>GHMEQTHRAIFRFVPRHEDELELEVDDPLLLELQAEDYWYEAYNMRTGARGVFPAYYAIEVTK[12x]

Aromatic residues cluster in the core of folded proteins, where they stabilize the structure through multiple interactions. NMR studies in the 1970s demonstrated that aromatic side chains can undergo ring flips—that is, 180° rotations of the χ2 dihedral angle (Cβ–Cγ axis)—even when engaged in stabilizing interactions in the hydrophobic core. Here we capture ring flipping events of a buried tyrosine residue in the SH3 domain of the JNK-interacting protein 1 (JIP1). Our data therefore suggest that the conformation of the aromatic ring at position 526 is determined by steric interactions dictated by the size of the surrounding amino acids.

The PCA suggests that a staggered conformation in group 2 is favoured over an eclipsed conformationin group 1 when residues with larger side chains are found in position 541, when isoleucine or leucine are occupying position 517 and when smaller residues are found in position 493. Accordingly, we designed four different mutants of JIP1-SH3 (H493A, V517A, V517L and A541L) and obtained their high-resolution structures by X-ray crystallography. Of note, three mutants (H493A, V517A and A541L) induce a staggered conformation of Y526, with χ2 dihedral angles ranging from −41° to −75°, whereas V517L shows an eclipsed conformation of Y526 and an almost identical structure to the wild-type protein. The high resolution of these structures, ranging from 1.4 to 1.9 Å, allows unambiguous determination of the conformation of Y526 and the surrounding residues, as demonstrated by their unbiased electron density maps.4-{[4-HYDROXY-PHENYL]-1H-BENZIMIDAZOLE-5-YL}-BENZIMIDAZOLE-2-YL-[4-HYDROXY-BENZENE] 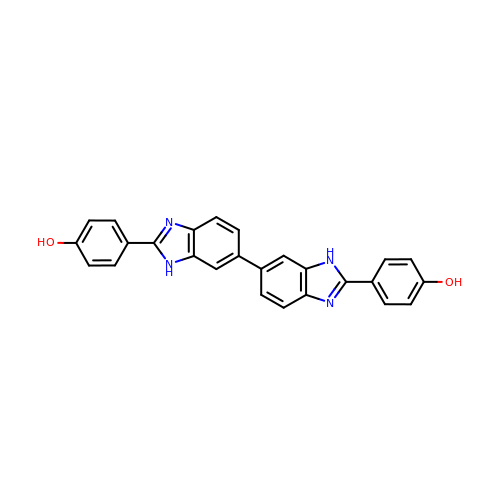| C26 H18 N4 O2 | LUIYJLIHLJLIPT-UHFFFAOYSA-N> SGSAGNGLVPSDPVLAETMKNERVVQDHNSALRGARPINFGYLIKDAELKLVQSIKGSLRGSKLPPGHKGAHGRVSKTNGS;> SMANTIKVEGYPSMEWPTSLDIPLKASEELVGIDLETDLPDDPTDLKTLLVEESSEKEHWLTIALAYCNHGKTNEGIRLIEMALDVFQNSERASLHTFLTWAHLNLAKGHSLSVETKEHELTQAELNLKDAIGFDPTWIGNMLATVELYYQRGHYDKALETSDLFVKSIHAEDHRSGRQSKPNCLFLLLRAKLLYQKKNYVASLKIFQELLVINPVLQPDPRIGIGLCFWQLKDPKMAIKSWQRALQINSKNTSAS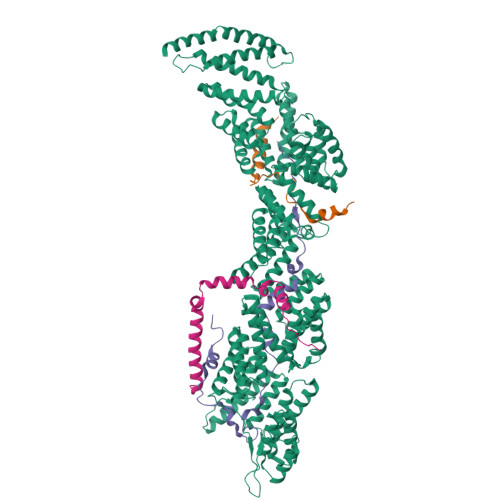ILVLLGEFHNSLTDSTNDEVFKETFSKALSDLKNIFSENQNNPVLLTLLQTYHYFKGDFQTVLDIYHHKILKMSPLIAKTVLSESSFWCGRAHYALGDYRKSFIMFQESLKKNEDNLMARLGLGQTQIKSNLLEESIITFENLYKTNESLQELNYILGLLYAGKTLDVKTSKSIPAKELNKLNEKALQYLERYIKLTVAKKNQLIISRVYLVISQLYESQNQYKISLDFLSKALEEMEFVNKDEVPLEILNNLACYHFINGDLTKADNLFEQAKAKVSDMNKSVNITLEYNIARTSEKTNWEKSESIYSQITSSHPSYISARIRNLYIKFAHSKINDSEMNIEINGLLEMNKSDLEMRSFYGWYLKNSEERKNSEKSTSHNKETLVKYNSHDAYALISLANLYVTIARDGKKSRNPKEQEKSKHSYLKAIQLYQKVLQIDPFNVFAAQGVAIIFAESKRLGPALEILRKIRDSLDNEDVQLNLAHCLLEMREFGKAIENYELVLKKFDNERTRPHILNLLGRAWYSRGMKERSVSFFQKALENAKTALELFVQQSAKNKFIHSVKFNIALLQFQIAETLRRSNPKFRTVQQIKDSLEGLEEGLALFKELNDLKEFNMIPKEELEQRIQLGETTMKSALERSLNEQEEFEKDQ;> SMSKKQEYIAPIKYQNSLPVPQLPPKLLAYPEAPETNPDSSQLINSLYVKTNISNLIQQDEDLGMPVDLMKFPGLLNKLDSKLLYGFDNVKLDKDDRILLRDPRIDRLTKT;> SKSDPFSRLKTRTKVYYQEIQKEENAKAKEMAQQEKLQEDRETKERREKELLLAQFRRLGGLERMIGELDIKFDFKF>[2x]SGAKPGKKTRGRVKIKMEFIDNKLRR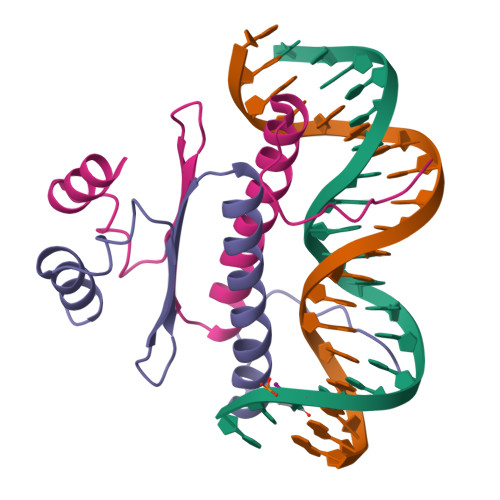YTTFSKRKTGIMKKAYELSTLTGTQVLLLVASETGHVYTFATRKLQPMITSETGKALIQTCLNSPD Sigma class glutathione transferases (Sigma GSTs) are key regulators of Th1 inflammatory responses, making them promising targets for development of therapies and vaccines. This study presents the first report on the crystallographic structures of recombinant 24-kDa sigma class GST from T. solium (rTs24GST), which were determined at resolutions of 1.30 and 1.75 Å. The structure of rTs24GST shows a typical GST folding with the thioredoxin domain in the small N-terminal α/β domain (residues 1–90), and the larger C-terminal comprising the α-helix domain (residues 91–212). Finally, a 24.3-kDa GST (Ts24GST) of medium abundance, belonging to the sigma class is principally expressed in the scolex and exhibits low activity against 1-chloro-2,4-dinitrobenzene (CDNB) compared to Ts25GST and Ts26GST. rTs24GST is an enzyme with low affinity for GSH.

Two crystallographic structures of rTs24GST without GSH (apo form) were determined at resolutions of 1.30 and 1.75 Å and analyzed. The second structure at 1.30 Å resolution was determinated using the rTs24GST 1.75 Å resolution coordinates as the initial model for MR. Moreover, this structure lacks the loop connecting alpha helices 4 and 5. The second region has the highest B-factor values in the overall structure and is located between residues Leu116 and His132 forming the loop connecting helices α4 and α5. In this region, the electron density is insufficient to build any model. The crystallographic structure corresponds to the apo form of a sigma class GST. These structures were determined in a C 2 2 21 space group (number 20), and in both cases, the asymmetric unit has a monomer with Wilson B-factor values below 21 Å2. However, the diffracted crystals obtained under GSH co-crystallization and soaking conditions did not show the GSH molecule bound to the protein. An analysis of the available space at the G-site in these crystallographic arrangements revealed minimal space for GSH to reach the site due to crystallographic contacts, which reduce or even prevent the success of crystal-soaking experiments with GSH.

> MDLQLKQAKLRLLYFNIRGRAELIRLVLNAAEKDFEDVRVSETEWPSLKSKMPFNQLPVLEVTTPNGQKVMLTESMAIARLLARTFGLYGDNAAEVYLIERMNSLTSSLLEEIYALGLKKVDSFKKLFEAEHLHEYMNAIEMALKERKSTFIAGPRVTLADLQVIVLIDTMNKFLPNTKHECKDKLDEIKEGVIRTKPGVARYLRSRPATDF> ITGQAACPESWIGFQRKCFYFSDDTKNWTSSQRFCDSQDADLAQVESFQELNFLLRYKGPSDHWIGLSREQGQPWKWINGTEWTRQFPILGAGECAYLNDKGASSARCYTERKWICSKSDIHVGTKHHHHHHHHG

Human LLT1 is a C-type lectin-like ligand of NKR-P1 (CD161, gene KLRB1), a C-type lectin-like receptor of natural killer cells. Similarly to mouse Clr-g, human LLT1 is a type II transmembrane glycoprotein which consists of an N-terminal cytoplasmic chain, transmembrane and stalk regions and a C-terminal CTL domain with two predicted N-linked glycosylation sites. The engagement of NKR-P1 on the NK cell with LLT1 on the target cell inhibits NK cell cytotoxicity and IFNγ production and contributes to NK self-tolerance in a similar way to the orthologous rodent NKR-P1B–Clr-b receptor–ligand pair. In this study, we present several structures of LLT1 under various conditions: monomeric (LLT1_mono), dimeric deglycosylated after the first N-acetyl­glucosamine unit (LLT1_D1 and LLT1_D2) and dimeric (packed into hexamers) with homogeneous GlcNAc2Man5 glycosylation (LLT1_glyco).

The monomeric form keeps the same fold with the exception of the position of an outer part of the long loop region. There is an important difference in the placement of the outer loop (residues 147–160) of the long loop region (residues 137–160). In LLT1_mono, residues 147–160 (the outer loop of the long loop region) are poorly visible and were not built in the deposited structure. A new conformation of the outer loop in the long loop region of a CTL receptor/ligand was observed; its newly observed position near α-helix 96–104 is probably the result of conformational sampling with satisfied packing positions of the neighbours and is without any special biological significance. The crystal packing of LLT1_mono was investigated to confirm that the form of the protein in this structure is really monomeric and that no possible partner participating in oligomer formation can be found among the symmetry-related copies. The classical dimerization interface is left open to the solvent, without any crystal contacts. The monomeric form of LLT1 was crystallized at pH 3.5 and the changed protonation state at low pH corresponds with the changed preferred intermolecular contacts and the formation of oligomers. As an example, residue His190, localized near the C-terminus in the dimerization interface, is charged at low pH and destabilizes this part of the interface. In LLT1_mono His190 is very likely to be protonated as it forms a hydrogen bond to the N-terminal Gln72 O of the same chain. Given that we observe standard dimers at pH 4.2 in the LLT1_glyco structure and only the extreme pH of 3.5 in LLT1_mono leads to dimer disruption, this direct observation of behaviour at extremely low pH is not relevant to normal biological limits.>MKFTVEREHLLKPLQQVSGPLGGRPTLPILGNLLLQVADGTLSLTGTDLEMEMVARVALVQPHEPGATTVPARKFFDICRGLPEGAEIAVQLEGERMLVRSGRSRFSLSTLPAADFPNLDDWQSEVEFTLPQATMKRLIEATQFSMAHQDVRYYLNGMLFETEGEELRTVATDGHRLAVCSMPIGQSLPSHSVIVPRKGVIELMRMLDGGDNPLRVQIGSNNIRAHVGDFIFTSKLVDGRFPDYRRVLPKNPDKHLEAGCD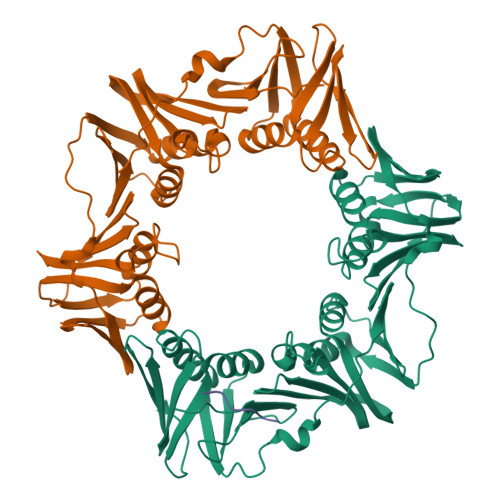LLKQAFARAAILSNEKFRGVRLYVSENQLKITANNPEQEEAEEILDVTYSGAEMEIGFNVSYVLDVLNALKCENVRMMLTDSVSSVQIEDAASQSAAYVVMPMRL[2x];> TLMTGQLGLF> TNLVAEPFAKLEQDFGGSIGVYAMDTGSGATVSYRAEERFPLCSSFKGFLAAAVLARSQQQAGLLDTPIRYGKNALVPWSPISEKYLTTGMTVAELSAAAVQYSDNAAANLLLKELGGPAGLTAFMRSIGDTTFRLDRWEL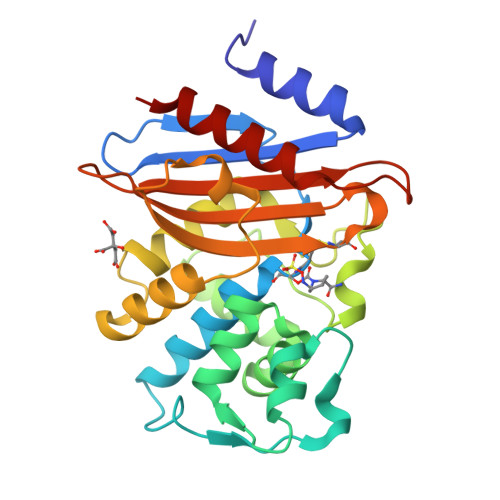ELNSAIPGDARDTSSPRAVTESLQKLTLGSALAAPQRQQFVDWLKGNTTGNHRIRAAVPADWAVGDKTGTCGVYGTANDYAVVWPTGRAPIVLAVYTRAPNKDDKHSEAVIAAAARLALEGLG>[2x]MMKNMILPIAFTALIASMTACSDETDPILTQKNWDGTATYFQSSDEHGFSMYYKPQVGFVGNPMPFYDPVAKDFKVMYLQDYRPNPEATYHPIFGVATKDGATYESLGELISCGGRDEQDAAIGTGGTIYNPADKLYYTFYTGNKFKPSSDQNAQVVMVATSPDFKTWTKNRTFYLKGDTYGYDKNDFRDPFLFQTEDGVYHMLIATRKNGKGHIAEFTSADLKEWESAGTFMTMMWDRFYECPDVFKMGDWWYLIYS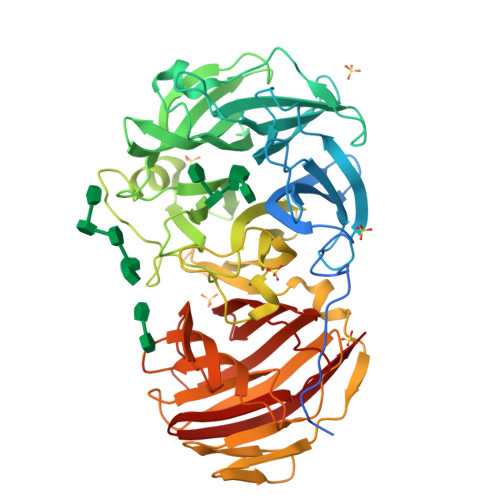EQASFMRKVQYFKGRTLEDLKATTANDAGIWPDNREGMLDSRAFYAGKTASDGTNRYIWGWCPTRAGNDNGNVGDVEPEWAGNLVAQRLIQHEDGTLTLGVPDAIDRKYTSAQEVKVMAKDGNMIESGKTYTLGEGASVIFNRLKVHNKISFTVKTASNTDRFGISFVRGTDSASWYSIHVNADEGKANFEKDGDDAKYLFDNKFNIPADNEYRVTIYSDQSVCVTYINDQLSFTNRIYQMQKNPWSLCCYKGEITVSDVQVSTY>MCPQKLTISWFAIVLLVSPLMAMWELEKDVYVVEVDWTPDAPGETVNLTCDTPEEDDITWTSDQRHGVIGSGKTLTITVKEFLDAGQYTCHKGGETLSHSHLLLHKKENGIWSTEILKNFKNKTFLKCEAPNYSGRFTCSWLVQRNMDLKFNIKSSSSSPDSRAVTCGMASLSAEKVTLDQRDYEKYSVSCQEDVTCPTAEETLPIELALEARQQNKYENYSTSFFIRDIIKPDPPKNLQMKPLKNSQVEVSWEYPDSWSTPHSYFSLKFFVRIQRKKEKMKETEEGCNQKGAFLVEKTSTEVQCKGGNVCVQAQDRYYNSSCSK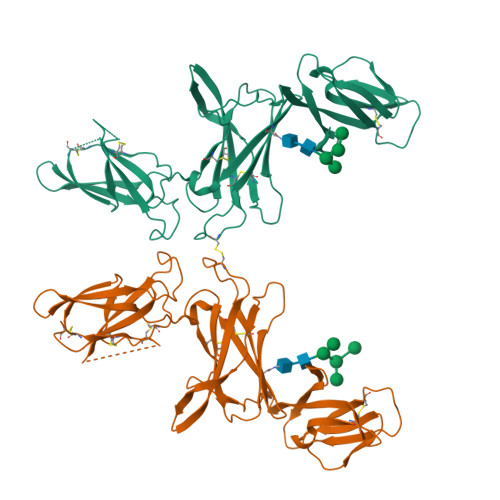WACVPCRVRSGTKHHHHHH[2x]> GSHMASMSKDEVKREAKDTDGNPEIKGERRRLHSEIQSGSLANNIKKSTVIVKN;> PTAIAICLYYKLGETPLPLVIETGK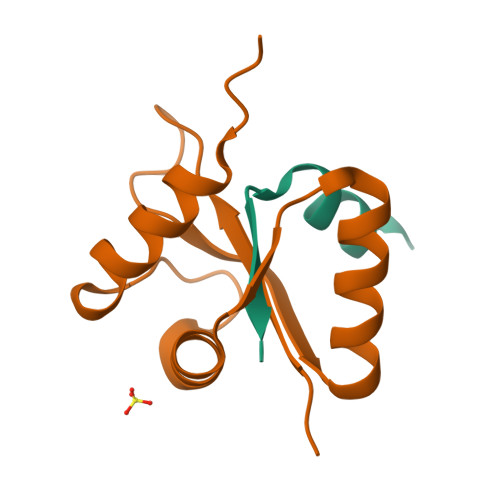DAKALQIIKLAELYDIPVIEDIPLARSLYKNIHKGQYITEDFFEPVAQLIRIAIDLDY> MKISENWLRTWVNPAIDSDTLSDQLTMLGLEVDELASVAKPFTGVVVGEVLTVEQHPDADRLRVTTVNIGSGEPLQIVCGAPNVRAGMKAPVATIGAVLPGDFKIKKGKLRGVESQGMLCGASEIDLEDKIDGLLELPADAPVGVNIREYLKLDDNVIDISITPNRGDCFSIRGIAREVAVINQLQMNEPEIKSVDATITDEKKVVINTDGAPRYLGRVIKNVNVKAATPEWMEQALARSGIRTHSILVDVTNYVLMELGQPMHAFDLAKIEGTVHVRQAKPQEKLQLLNDQEVELQEDVMVIADDQKALAIAGIMGGLASSVTDDTTDIFLESAFFAPLAIAGRARRFGLHTDSSQRYERGVDFELPVIAMNRASQLIQELAGGEFGPITVAEKSDLLPKREAIELKQAQVDQLLGYKVAAEFITDALTRLGCEVTVQANGEWSVVPPSHRYDMAIYQDLIEEVARIDGYDNIQISLPSMDVQLAKYQDRFEIAQLRQTVATLGYQEAISFSFADAKLEKQLNPQVSPLMLANPISSDLAAMRSTLLSSLIPCVQYNLNRQQSRVRFFELGLRFDYQNANSIQDLKQIPTLALVAVGSREPESWHAKPQPMDFFDFKGEVEEILAAGRVKV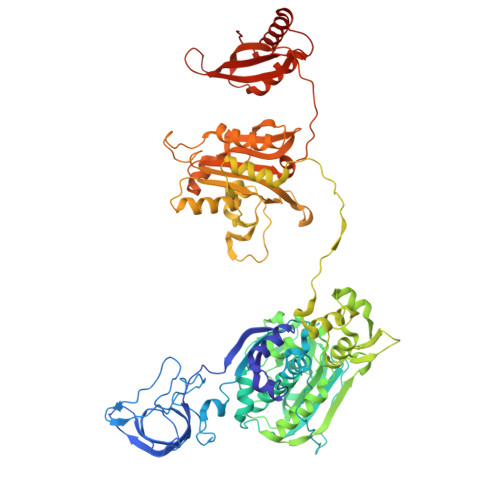EYVRSERPWLHPGQSAEILVDGQSIGYLGRLHPSLENELDLSTTWVAELDQAAVLQSYVSNFTELSRFPSVRRDIALLISDNINVRDIQQLIEKTGGELLDSTWLFDVYTGQGVEEGKRSLAFALLWQHPSRTLEDAEIKSGMDNIIQVLENTYQATLRAS>[8x]MDKFRMMFQFLQSNQESFMNGICGIMALASAQMYSSFEFSCPCMPEYNYTYGIGLLIIPPIWFFLLGFVLNNNVSVLAEEWKRPTGRRTKDPSVLRYMLCSITQRSLIAPAVWVSVTLMDGKSFLCAFSINLDIEKFGNASLVIGMTETEKLKFLARIPCKDLFEDNEVRVAATRYIKCISQACGWMFLLMMTFTAFLIRAIRPCFTQAA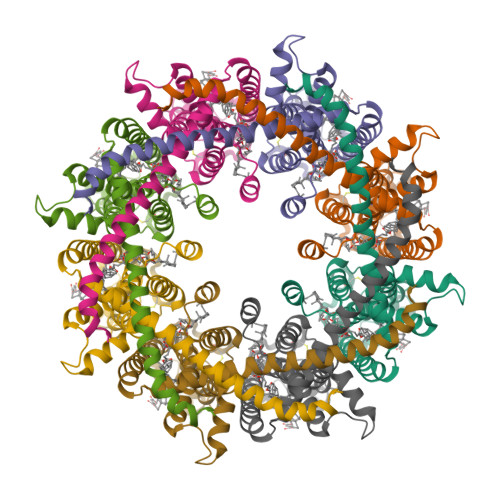FLKTKYWSHYIDIERKMFDETCKEHAKSFAKVCIHQYFENISGEMQNFHRHQSKDTSDAEEEEKQRSDEDKLLGIKAQEDMNKVLENLYFQ>[2x]MSQPRTPEQALDTPGDCPPGRRDEDAGEGIQCSQRMLSFSDALLSIIATVMILPVTHTEISPEQQFDRSVQRLLATRIAVYLMTFLIVTVAWAAHTRLFQVVGKTDDTLALLNLACMMTITFLPYTFSLMVTFPDVPLGIFLFCVCVIAIGVVQALIVGYAFHFPHLLSPQIQRSAHRALYRRHVLGIVLQGPALCFAAAIFSLFFVPLSYLLMVTVILL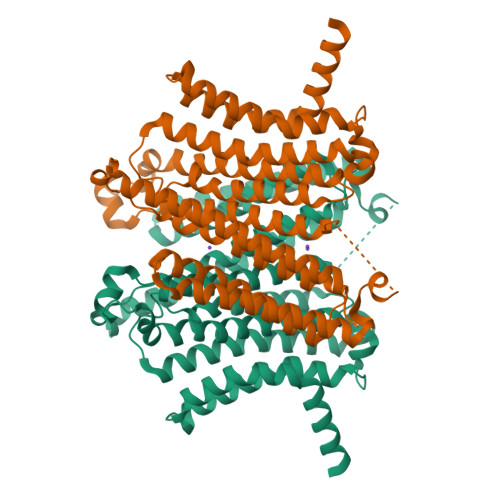PYVSKVTGWCRDRLLGHREPSAHPVEVFSFDLHEPLSKERVEAFSDGVYAIVATLLILDICEDNVPDPKDVKERFSGSLVAALSATGPRFLAYFGSFATVGLLWFAHHSLFLHVRKATRAMGLLNTLSLAFVGGLPLAYQQTSAFARQPRDELERVRVSCTIIFLASIFQLAMWTTALLHQAETLQPSVWFGGREHVLMFAKLALYPCASLLAFASTCLLSRFSVGIFHLMQIAVPCAFLLLRLLVGLALATLRVLRGLARPEHPPPAPTGQDDPQSQLLPAPC>MMKVLIVESEFLHQDTWVGNAVERLADALSQQNVTVIKSTSFDDGYAILSANEAIDCLMFSYQMEQPDEHLSVRQLIGKLHERQQNVPVFLLGDREKATASLDRDLLELVDEFAWILEDTADFIAGRAVAAMTRYRQQLLPPLFNALMKYSDIHEYSWAAPGHQGGVGFTKTPSGRFYHDYYGENLFRSDMGIERTTLGSLLDHTGAFGESEKNAARVFGADRSWSVVVGTSGSNRTIMQACMTDNDVVVLDRNCHKSIEQGLILTGAKPVYMVPSRNRYGIIGPIYPQEMQPETLQKKISASPLTKTKAGQKPSYSVVTNCTYDGVCYNAKEAQDLLAKTSDRIHFDEAWYGYARFNPIYCDHYAMRGEPGDHNGPTVFATHSTHKLLNALSQASYIHVREGRGAVNFSRFNQAYMMHATTSPLYAICASNDVAVSMMDGNSGLSLTQEVIDEAVDFRQAMARLYKEFTDEGDWFFKPWNKDVVTDPQTGKTYDFADAPAKLLATDQNCWVMRPGETWHGFKDLPDNWSMLDPIKVSILAPGMGDDGELEASGVPAALVTAWLGRHGIVPTRTTDFQIMFLFSMGVTRGKWGTLINTLCSFKHHYDANTPLAQVMPELVQDYPDTYANMGIHDLGDKMFAWLRENNPGARLNAAYSTLPVAEITPRDAYNAIVNNNIEMVAIENLPGRIAANSVIPYPPGIPMLLSGENFGDENSPQVGYLRSLQSWDHHFPGF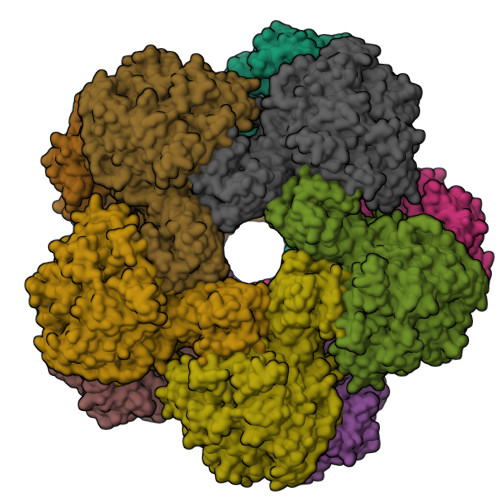EHETEGTEIIDGVYHVMCVKA[10x]>[10x]GHMSIPFTRWPEEFARRYREKGYWQDLPLTDILTRHAASDSI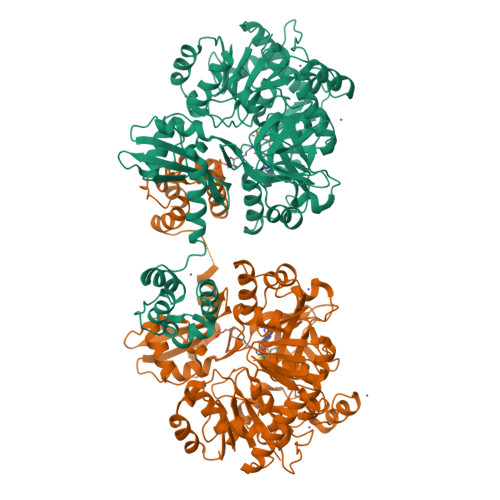AVIDGERQLSYRELNQAADNLACSLRRQGIKPGETALVQLGNVAELYITFFALLKLGVAPVLALFSHQRSELNAYASQIEPALLIADRQHALFSGDDFLNTFVTEHSSIRVVQLLNDSGEHNLQDAINHPAEDFTATPSPADEVAYFQLSGGTTGTPKLIPRTHNDYYYSVRRSVEICQFTQQTRYLCAIPAAHNYAMSSPGSLGVFLAGGTVVLAADPSATLCFPLIEKHQVNVTALVPPAVSLWLQALIEGESRAQLASLKLLQVGGARLSATLAARIPAEIGCQLQQVFGMAEGLVNYTRLDDSAEKIIHTQGYPMCPDDEVWVADAEGNPLPQGEVGRLMTRGPYTFRGYYKSPQHNASAFDANGFYCSGDLISIDPEGYITVQGREKDQINRGGEKIAAEEIENLLLRHPAVIYAALVSMEDELMGEKSCAYLVVKEPLRAVQVRRFLREQGIAEFKLPDRVECVDSLPLTAVGKVDKKQLRQWLASRASAGRASIPASKAALREVILPLLDESDEPFDDDNLIDYGLDSVRMMALAARWRKVHGDIDFVMLAKNPTIDAWWKLLSREVK>[4x]SHGMAVTKVTVDGIEFPPTITPPGSSKSLTLLGAGVRGIEIETIQIKVTAIGVYAEPEVIASHLQKWKGKSASELVEDDGFFKDLVQAPVEKLVKITMIK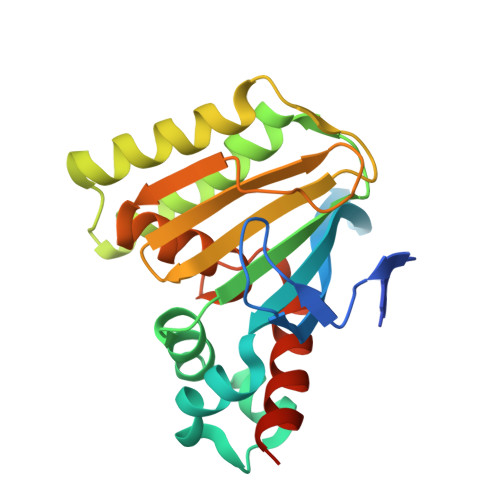GLKGSQYGGAVEENIRDRLAALDKYSEAEEEALEEFREFFKTKSLPKGSVIFFHWPSPSTLQISFSTDGSLPEEAEATVENANVAAALLGVFLGENSVSPSTKASVAEGISALLMKNKDEKEV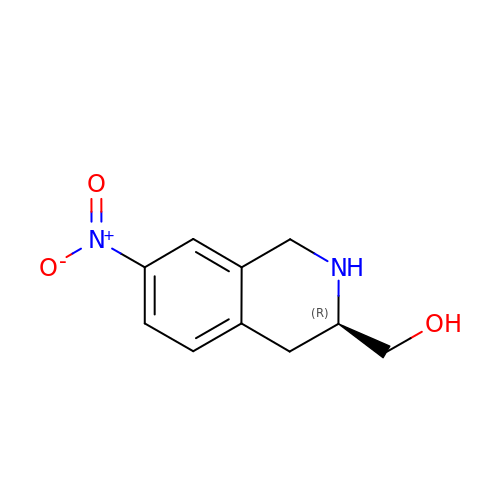[(3R)-7-NITRO-1,2,3,4-TETRAHYDROISOQUINOLIN-3-YL]METHANOL | C10 H12 N2 O3 | RNUCRXHRBPLYTA-SECBINFHSA-N> MGSSHHHHHHASDPVNPEKLLVITVATAETEGYLRFLRSAEFFNYTVRTLGLG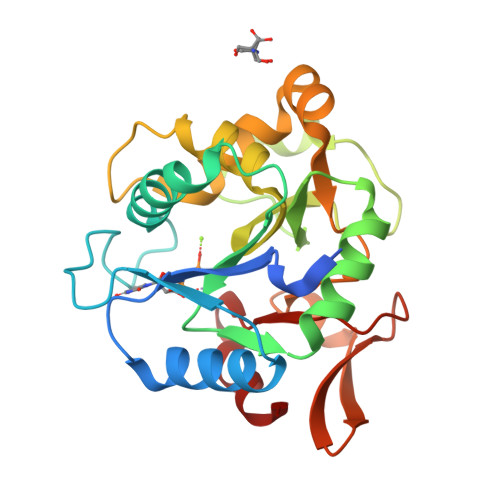EEWRGGDVARTVGGGQKVRWLKKEMEKYADREDMIIMFVDSYDVILAGSPTELLKKFVQSGSRLLFSAESFCWPEWGLAEQYPEVGTGKRFLNSGGFIGFATTIHQIVRQWKYKDDDDDQLFYTRLYLDPGLREKLSLNLDHKSRIFQNLNGALDEVVLKFDRNRVRIRNVAYDTLPIVVHGNGPTKLQLNYLG> MADTQYILPNDIGVSSLDSREAFRLLSPTERLYAYHLSRAAWYGGLAVLLQTSPEAPYIYALLSRLFRAQDPDQLRQHALAEGLTEEEYQAFLVYAA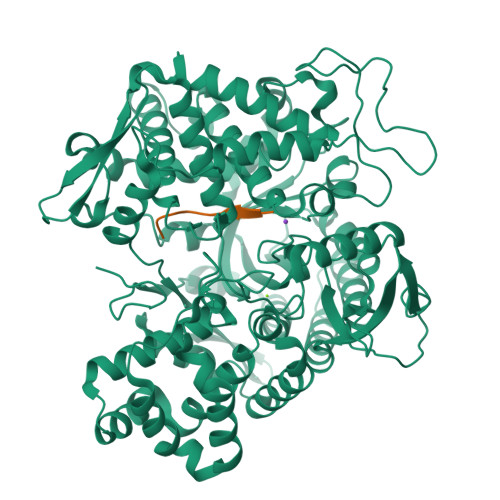GVYSNMGNYKSFGDTKFVPNLPKEKLERVILGSEAAQQHPEEVRGLWQTCGELMFSLEPRLRHLGLGKEGITTYFSGNCTMEDAKLAQDFLDSQNLSAYNTRLFKEVDGCGKPYYEVRLASVLGSEPSLDSEVTSKLKSYEFRGSPFQVTRGDYAPILQKVVEQLEKAKAYAANSHQGQMLAQYIESFTQGSIEAHKRGSRFWIQDKGPIVESYIGFIESYRDPFGSRGEFEGFVAVVNKAMSAKFERLVASAEQLLKELPWPPTFEKDKFLTPDFTSLDVLTFAGSGIPAGINIPNYDDLRQTEGFKNVSLGNVLAVAYATQREKLTFLEEDDKDLYILWKGPSFDVQVGLHALLGHGSGKLFVQDEKGAFNFDQETVINPETGEQIQSWYRCGETWDSKFSTIASSYEECRAESVGLYLSLHPQVLEIFGFEGADAEDVIYVNWLNMVRAGLLALEFYTPEAFNWRQAHMQARFVILRVLLEAGEGLVTITPTTGSDGRPDARVRLDRSKIRSVGKPALERFLRRLQVLKSTGDVAGGRALYEGYATVTDAPPESFLTLRDTVLLRKESRKLIVQPNTRLEGSDVQLLEYEASAAGLIRSFSERFPEDGPELEEILTQLATADARFW;> DRVYIHPF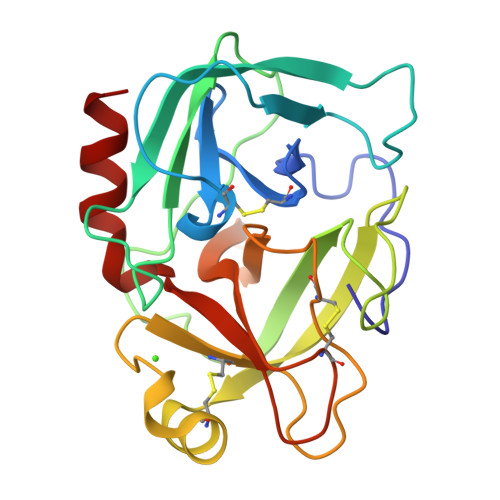> VVGGTRAAQGEFPFMVRLSMGCGGALYAQDIVLTAAHCVSGSGNNTSITATGGVVDLQSGAAVKVRSTKVLQAPGYNGTGKDWALIKLAQPINQPTLKIATTTAYNQGTFTVAGWGANREGGSQQRYLLKANVPFVSDAACRSAYGNELVANEEICAGYPDTGGVDTCQGDSGGPMFRKDNADEWIQVGIVSWGYGCARPGYPGVYTEVSTFASAIASAARTL>MFSTPLPAELRPLLERLLTLAQDELSGGDLETFSLRLERYLPDLHAGLTAVYPDAEGLLERLLPILTAAHQARSADLRRLDAKRLLAPDWFQRPEMIAYVAYTERFAGTLRGVEERIDYLEELGVRYLHLMPFLKPRPAPHDGGYAVMDYRAVREDLGTMADL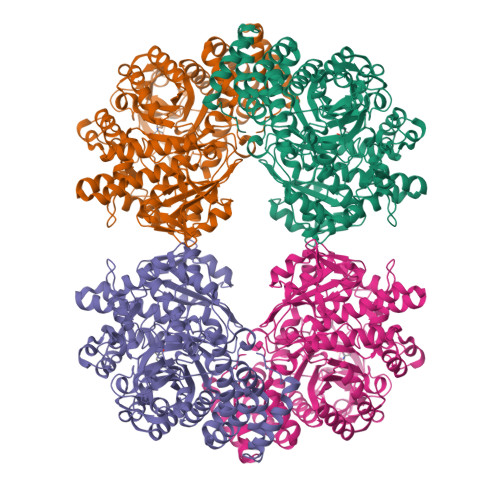EALTAKLRARGIALCCDLVLNHVAQEHEWALRARRGEAKYQRYFHMFPDRTLPDEYEKTLPEVFPDFAPGNFTFDEESGQWVWTTFNRWQWDLNWANPEVFLEFADLILWLANRGVEVFRLDAIAFIWKRLGTNCQNQPEVHAITQALRAVARIVAPAVLFKAEAIVAPDDLIHYLGQGPHFGLLSDTAYHNSLMVQIWSSLASRDVRLMSEALRRFPLKPTNTAWCTYLRCHDDIGWAIADEDAARVGLSGEAHRRFLSDYYSGRFPASFSRGLVFQENPRTGDRRISGSAASLAGLEQALERGDPHQLHLSLERLLLGHAVVLGFGGIPLLYMGDELALLNDHSYLEEPEHAEDNRWVHRPHMDWEKAARAKADPTSPEGRMYHGLRHLIRVRRTTPHFHAALEAQILEPRNPHVFGYVRRHPLGNLVALYNFSEEVQYYPAEVLWQQGLGLPFDRISGQLVPIEHHLVRLEPYARLWITDESDRHHHHHH[4x]> NECISVKGRIYSILKQIGSGGSSKVFQVLNEKKQIYAIKYVNLEEADNQTLDSYRNEIAYLNKLQQHSDKIIRLYDYEITDQYIYMVMECGNIDLNSWLKKKKSIDPWERKSYWKNMLEAVHTIHQHGIVHSDLKPANFLIVDGMLKLIDFGIANQMQPDT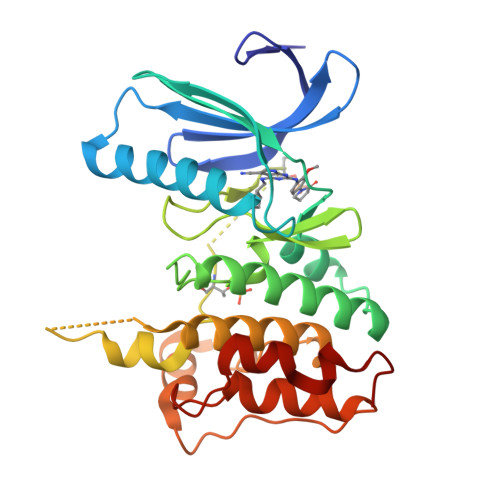TSVVKDSQVGTVNYMPPEAIKDMSSSRENGKSKSKISPKSDVWSLGCILYYMTYGKTPFQQIINQISKLHAIIDPNHEIEFPDIPEKDLQDVLKCCLKRDPKQRISIPELLAHPYVQIQTLE> GDNQDRTVANTQPSGPSNSTEIPALTAVETGHTSQVDPSDTIQTRHVVNFHSRSESTIENFMGRAACVFMDQYKINGEETSTDRFAVWTINIREMAQLRRKCEMFTYMRFDIEMTMVITSCQDQGTILDQDMPVLTHQIMYVPPGGPIPAKVDGYEWQTSTNPSVFWTEGNAPPRISIPFISVGNAYSSFYDGWSHFTQDGTYGYTTLNAMGKLYIRHVNRSSPHQITSTIRVYFKPKHIKAWVPRPPRLCPYINKRDVNFVVTEITDSRTSITDTPHPEHSVLATH;> SPSAEECGYSDRVRSMTLGNSTITTQESANVVVGYGEWPSYLSDREATAEDQPTQPDVATCRFYTLESVQWEKTSPGWWWKFPEALKNMGLFGQNMHYHYLGRAGYTIHVQCNASKFHQGCLLVVCVPEAEMGCADTDTTFPATELTTEDTPHVFTSDSITGKKVQAAVCNAGMGVGVGNLTIFPHQWINLRTNNSATIVIPYINSVPMDNMFRHYNFTLMIIPFAPLNFTDGATAYVPITVTIAPMYAEYNGLRLASTQ;> GVPVLNTPGSNQFLTSDDYQSPSAMPQFDETPEMHIPGEVRNLMEIAEVDSVVPVNNVTGKTKSMDAYQIPVGTGNTDKTKPIFSFQMDPGYSSVLKRTLLGEMLNYYAHWSGSVKLTFLFCGSAMATGKLLISYSPPGASVPTSRKDAMLGTHIVWDIGLQSSCVLCVPWISQSHYRMVQQDPYTSAGYITCWYQTNIVVPPGAPTSCDVLCFASACNDFSVRLLRDTPFMAQPGKLQ;> MGAQVSTQKTGAHETSLSAKGNSIIHYTNINFYKDAASSASNRQDIQQDPGKFTDPVKDLMIKTLPALN

Viruses from the family Picornaviridae form non-enveloped icosahedral virions that are about 30 nm in diameter. The capsid proteins VP1, VP2, VP3, and VP4 originating from a single polyprotein form a protomer, the basic building block of the icosahedral capsid. The entire capsid consists of 60 such protomers, arranged in 12 pentamer units. Here we show that the exit of the RNA from the particles of echoviruses 18 and 30 requires capsid opening and results in a loss of up to three adjacent capsid protein pentamers.

We did not detect native echovirus 18 virions that lacked pentamers at neutral pH. The electron density of the genomes is distributed uniformly in echovirus 18 virions at neutral pH, but transforms to a grainy appearance in activated particles at acidic pH. The inter-pentamer contacts of 11,000 Å2 in native echovirus 18 virion are reduced to 5400 Å2 in the activated particles. Correspondingly, the interaction between two pentamers in an activated particle of echovirus 18 is 25% weaker than that in a native virion. Comparing the cryo-EM images of native virions with activated particles of echovirus 18, as well as other enteroviruses, reveals that their genomic RNAs undergo conformational changes upon exposure to acidic pH.> GAAAGVAAWLPFARAAAIGWM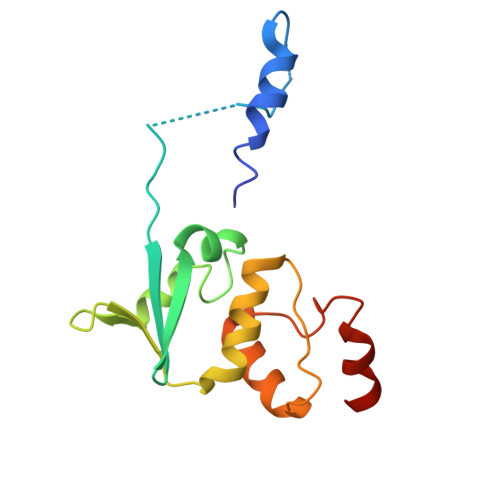PVANCPMPLAPADKNKRQDELIVLNVSGRRFQTWRTTLERYPDTLLGSTEKEFFFNEDTKEYFFDRDPEVFRCVLNFYRTGKLHYPRYECISAYDDELAFYGILPEIIGDCCYEEYKDRKREN>GSSHHHHHHSSGLVPRGSHMGSIIDAAAAADPVVLMETAFRKAVKSRQIPGAVIMARDASGNLNYTRCFGARTVRRDENNQLPPLQVDTPCRLASATKLLTTIMALQCMERGLVDLDETVDRLLPDLSAMPVLEGFDDAGNARLRERRGKITLRHLLTHTSGLSYVFLHPLLREYMAQGHLQSAEKFGIQSRLAPPAVNDPGAEWIYGANLDWAGKLVERATGLDLEQYLQENICAPLGITDMTFKLQQRPDMLARRADQTHRNSADGRLRYDDSVYFRADGEECFGGQGVFSGPGSYMKVLHSLLKRDGLLLQPQTVDLMFQPALEPRLEEQMNQHMDASPHINYGGPMPMVLRRSFGLGGIIALEDLDGENWRRKGSLTFGGGPNIVWQIDPKAGLCTLAFFQLEPWNDPVCRDLTRTFEHAIYAQ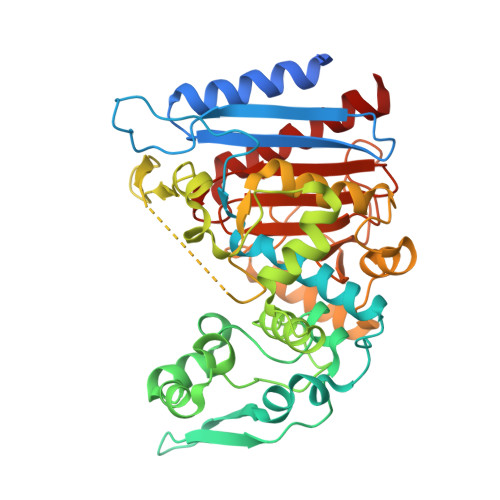YQQG[4x]>GGSGERKISRIHLVSEPSITHFLQVSWEKTLESGFVITLTDGHSAWTGTVSESEISQEADDMAMEKGKYVGELRKALLSGAGPADVYTFNFSKESCYFFFEKNLKDVSFRLGSFNLEKVENPAEVIRELICYCLDTTAENQAKNEHLQKELEHEEGKILRAQLEFNQIKAEIERKLAEKDEEMEQAKRNHLRVVD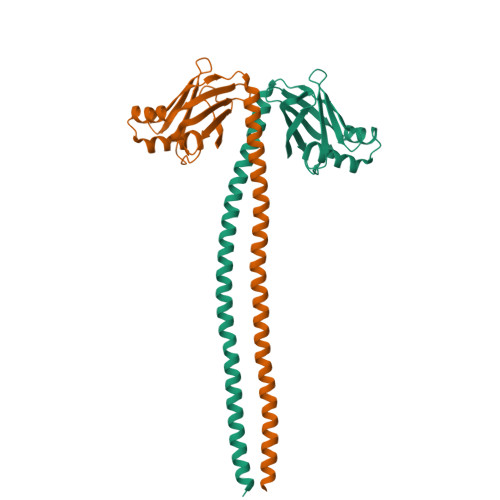SLQTSLDAETRSRN[2x]> MKERILQEIKTRVNRKSWELWFSSFDVKSIEGNKVVFSVGNLFIKEWLEKKYYSVLSKAVKVVLGNDATFEITYEAFEPHSSYSEPLVKKRAVLLTPLNPDYTFENFVVGPGNSFAYHAALEVAKHPGRYNPLFIYGGVGLGKTHLLQSIGNYVVQNEPDLRVMYITSEKFLNDLVDSMKEGKLNEFREKYRKKVDI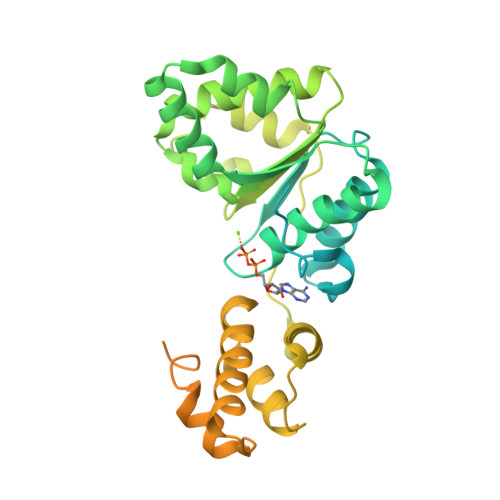LLIDDVQFLIGKTGVQTELFHTFNELHDSGKQIVICSDREPQKLSEFQDRLVSRFQMGLVAKLEPPDEETRKSIARKMLEIEHGELPEEVLNFVAENVDDNLRRLRGAIIKLLVYKETTGKEVDLKEAILLLKDFIKPNRVKAMDPIDELIEIVAKVTGVPREEILSNSRNVKALTARRIGMYVAKNYLKSSLRTIAEKFNRSHPVVVDSVKKVKDSLLKGNKQLKALIDEVIGEISRRALSG> MMNDIAHNLAQVRDKISAAATRCGRSPEEITLVAVSKTKPASAIAEAIDAGQRQFSEHYVQEGVDKIRHFQELGVTGLEWNFAGPLQSNKSRLVAEHFDWCITIDRLRIATRLNDQRPAELPPLNVLIQINISDENSKSGIQLAELDELAAAV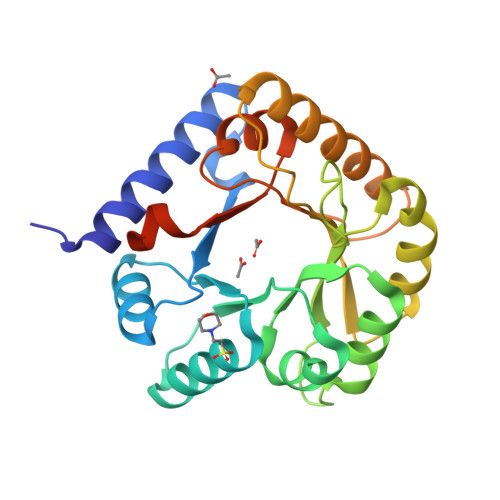AELPRLRLRGLSAIPAPESEYVRQFEVARQMAVAFAGLKTRYPHIDTLALGQSDDMEAAIAAGSTMVAIGTAIFGARDYSKKGSLEHHHHHH>SNAMDVQLPIEAKDIQKLIPHRYPFLQLDRITAFEPMKTLTAIKNVSINEPQFQGHFPDLPVMPGVLIIEAMAQACGTLAILSEGGRKENEFFFFAGIDEARFKRQVIPGDQLVFEVELLTSRRGIGKFNAVAKVDGQVAVEAIIMCAKR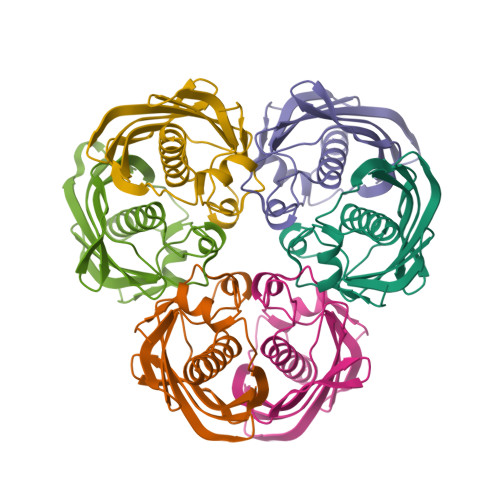VV[6x]> MLYSNLINVKQKVISIREKLGDPRL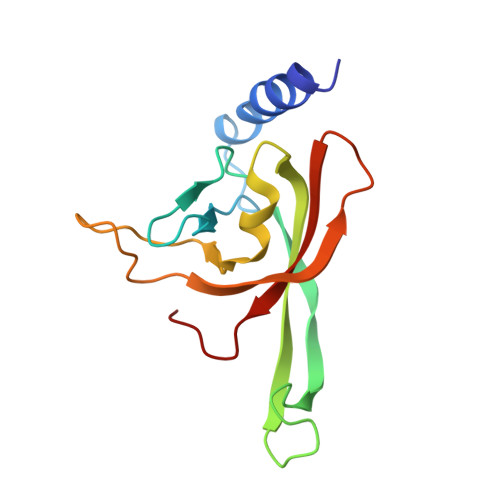KSLVFEYPAGQLFRVTPKLKVSMVPKNMIGLPLDSKSNITISADDYYITDVSRNVPEAAFRTRAWLDPVINDSGVIVSGINCRCHVINDKSGLSYDLILRKEREVRV> TCGTCA;> GAACGACATTGACGAGGAGTC;> TCGAGTCC;> ATGTCGT

In this work, we exhaustively probe the ability of all 36 immobile HJ sequences to form DNA crystals in two different designed systems. Three separate self-assembling DNA crystal systems are described in this report: the “4 × 5” and “4 × 6” designs (collectively referred to as the 4 × N systems), and a third construct with a “scrambled” sequence variant of the 4 × 6 lattices. Self-assembly was mediated by three constituent oligonucleotides: (S1) containing four sequence repeats of either 5 or 6 bases; (S2) composed of 21 bases containing complementary regions to both (S1); and (S3) which forms the second junction crossover. The HJ serves as the fundamental component at the core of each unit, and the ultimate assembly of the full lattice is facilitated by the complementary 2-base sticky ends that tail each duplex.

Each asymmetric unit could be defined as either a HJ containing 10 and 11 bp on each arm, or as a 21-bp linear duplex. Because the 4 × 6 system yielded R3 symmetry in 5 of 17 junctions, we considered whether the downstream sequences adjacent to the junction could play a role in crystallization efficiency, junction angle, and symmetry preference, or if the HJ alone was the singular determinant. To investigate this possibility, we designed “scrambled” sequences with targeted base substitutions, while maintaining GC content, along each “stem”. Contrary to the buffer preference observed with the native P32 crystals, the scrambled systems exhibited an exclusive preference towards low salt buffers, much like the native R3 crystals. Remarkably, only J1 and J2 retained the P32 symmetry, with all others yielding an R3 lattice. There appeared to be only a marginal difference in the average cell lengths in the R3 scramble crystals (a = b = 113.04 c = 51.10) relative to the native 4 × 6 sequences: the a, b axis trended ~2 Å shorter and c ~1.3 Å longer, whereas in the J1 and J2 cases, the crystals were in good agreement with the original 4 × 6 motif. The average angles of the R3 and P32 crystals were 61.00° (σ = 1.21) and 58.05° (σ = 1.39), respectively. However, in the majority of the crystal structures reported here, the cacodylate anion indeed fits best into the electron density map of our X-ray structures, due to the presence of sodium cacodylate in the crystallization solution.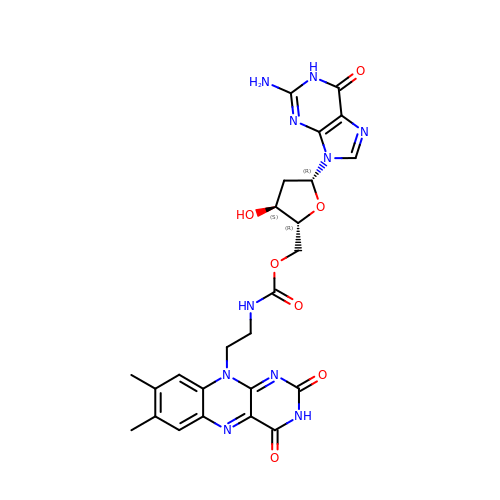2'-deoxy-5'-O-{[2-(7,8-dimethyl-2,4-dioxo-3,4-dihydrobenzo[g]pteridin-10(2H)-yl)ethyl]carbamoyl}guanosine | C25 H26 N10 O7 | JIELMHTXDVQHJI-ARFHVFGLSA-N4-{2-[(cyclohexylmethyl)amino]ethyl}-2-[(2-phenylethyl)amino]-3,7-dihydro-8H-imidazo[4,5-g]quinazolin-8-one 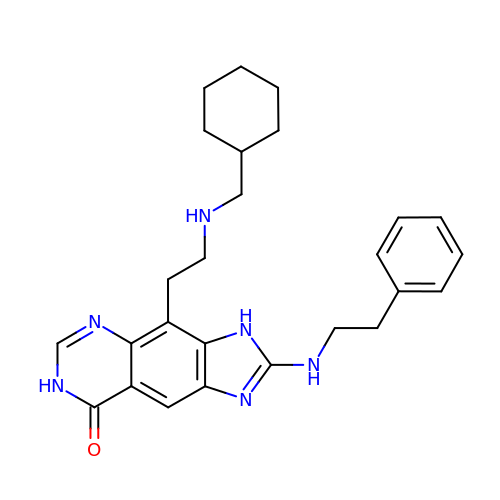| C26 H32 N6 O | WJSLFMAXPWEECW-UHFFFAOYSA-N> GHMELKREEITLLKELGSGQFGVVKLGKWKGQYDVAVKMIKEGSMSEDEFFQEAQTMMKLSHP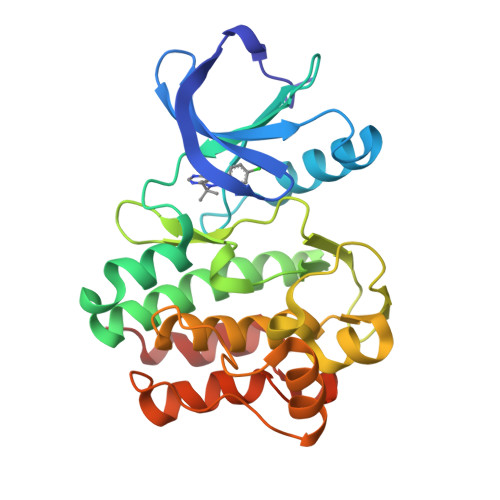KLVKFYGVCSKEYPIYIVTEYISNGCLLNYLRSHGKGLEPSQLLEMCYDVCEGMAFLESHQFIHRDLAARNCLVDRDLCVKVSDFGMTRYVLDDQYVSSVGTKFPVKWSAPEVFHYFKYSSKSDVWAFGILMWEVFSLGKMPYDLYTNSEVVLKVSQGHRLYRPHLASDTIYQIMYSCWHELPEKRPTFQQLLSSIEPLREKDKH> THSQLDQLLTGLVDRVAEVDHAVVLSEDGLVVSKSTGFLRDDAERLA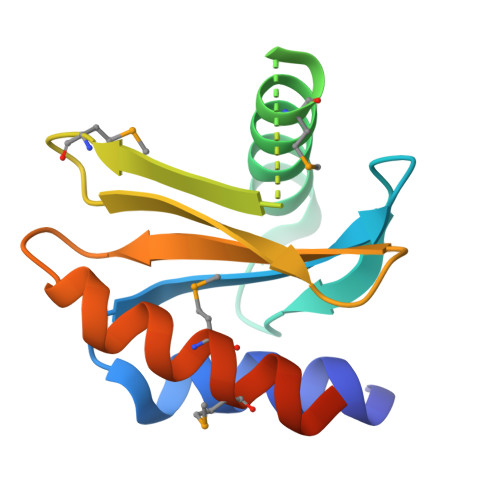ATASGLMSLSKGVSMDFRRGPVRQALIEMGKGYLILTAAGPGAHLVVLTRQGADVGVVAYQMNMLVKKIGEHLSAPPRG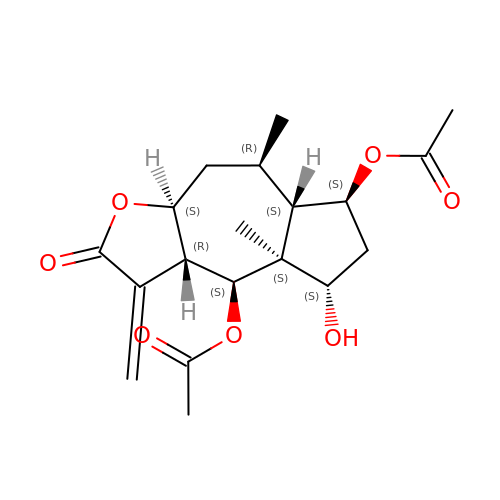[(3aS,5R,5aS,6S,8S,8aS,9S,9aR)-9-acetyloxy-8-hydroxy-5,8a-dimethyl-1-methylidene-2-oxo-4,5,5a,6,7,8,9,9a-octahydro-3aH-azuleno[6,5-b]furan-6-yl] acetate | C19 H26 O7 | JXEGMONJOSAULB-IZZBGLMFSA-N> IVGGQECKDGECPWQALLINEEN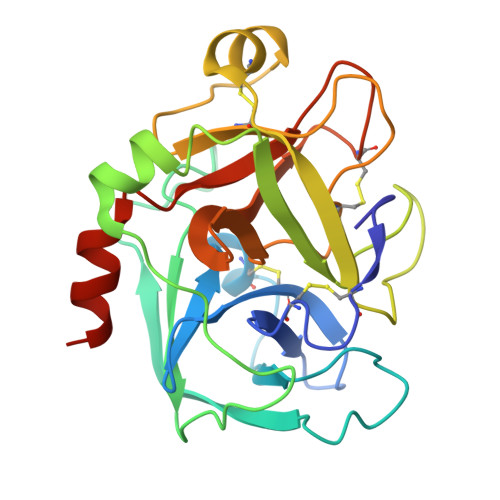EGFCGGTILSEFYILTAAHCLYQAKRFKVRVGDRNTEQEEGGEAVHEVEVVIKHNRFTKETYDFDIAVLRLKTPITFRMNVAPACLPERDWAESTLMTQKTGIVSGFGRTHEKGRQSTRLKMLEVPYVDRNSCKLSSSFIITQNMFCAGYDTKQEDACQGDSGGPHVTRFKDTYFVTGIVSWGEGCARKGKYGIYTKVTAFLKWIDRSMKTRGLP[[(2~{R},3~{S},4~{R},5~{R})-5-(6-aminopurin-9-yl)-3,4-bis(oxidanyl)oxolan-2-yl]methoxy-oxidanyl-phosphoryl] (2~{S})-2-azanyl-4-methyl-pentanoate | C16 H25 N6 O8 P | 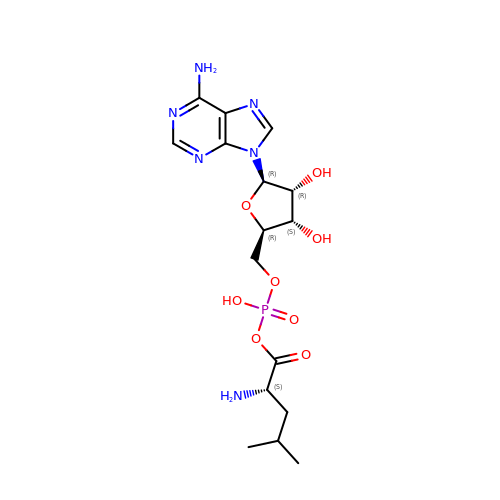AXWPLGAOCISUCB-OPYVMVOTSA-N>EFGMTYYRVVLIGEQGVGKSTLANIFAGVHDSMDSDCEVLGEDTYERTLMVDGESATIILLDMWENKGENEWLHDHCMQVGD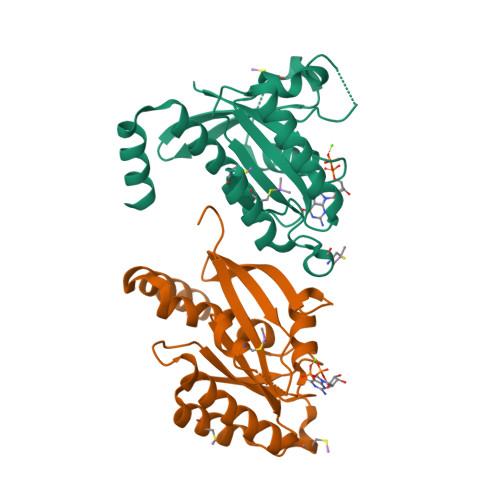AYLIVYSITDRASFEKASELRIQLRRARQTEDIPIILVGNKSDLVRCREVSVSEGRACAVVFDCKFIETSAAVQHNVKELFEGIVRQVRLRRDSKEKNERRLAYQKRKES[2x]6,7-dimethoxy-2-methyl-~{N}-[(1~{R})-1-[3-(trifluoromethyl)phenyl]ethyl]quinazolin-4-amine 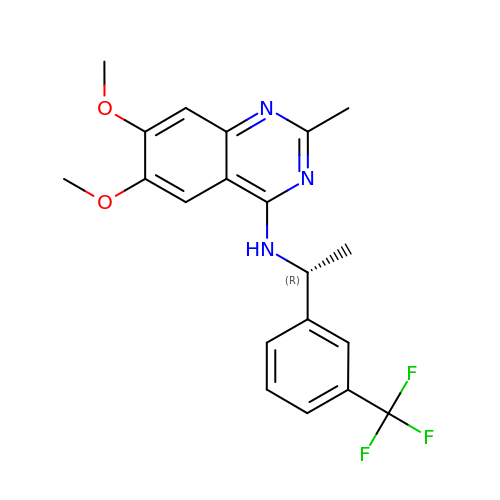| C20 H20 F3 N3 O2 | UWEJNKMEGIGAGY-LLVKDONJSA-N> GAEPYGQKKFIEIAGKRMAYIDEGEGDPIVFQHGNPTSSYLWRNIMPHLEGLGRLIACDLIGMGDSDKLSPSGPDRYSYAEHRDYLFALWEALDLGDNVVLVIHDWGSALGFDWANQHRDRVQGIAYMEAIVTPLEWADWPEEVRDIFQGFRSPAGEEMVLENNIFVERVLPGAILRQLSDEEMAEYRRPFLNAGEDRRPTLSWPRQIPIDGEPADVVAIVSDYASWLAESDIPKLFINAEPGAIVTGRMRDFCRSWPNQTEITVKGAHFIQEDSPDEIGAAIAEFVRRLRVAAGV

Haloalkane dehalogenases (HLDs) (EC 3.8.1.5) are hydrolytic enzymes that cleave carbon-halogen bonds in a broad range of halogenated aliphatic compounds, resulting in a corresponding alcohol, a halide ion, and a proton. The tertiary structure of HLDs is comprised of two domains: an α/β-hydrolase core domain and a helical cap domain. HLDs are divided into three subfamilies, HLD-I, HLD-II, and HLD-III, according to the composition of their catalytic residues and the anatomy of the cap domain. Based on the sequences of modern haloalkane dehalogenases from the subfamily II, the most common ancestor of thoroughly characterized enzymes LinB from Sphingobium japonicum UT26 and DmbA from Mycobacterium bovis 5033/66 was in silico predicted, recombinantly produced and structurally characterized.

The ancestral enzyme AncLinB-DmbA was crystallized using the sitting-drop vapor-diffusion method, yielding rod-like crystals that diffracted X-rays to 1.5 Å resolution. The structural organization of AncLinB-DmbA is similar to other HLDs-II subfamily members; it is composed of two compact domains, a cap domain and a main domain. The catalytic triad contains nucleophile D109, catalytic acid E133, and catalytic base H273. W110 and N39 act as halide-stabilizing residues in AncLinB-DmbA. The chloride anion is coordinated by two halide stabilizing residues with distances between the Nε1 atom in W110 and the Nδ1 atom in N39 of 3.29 and 3.37 Å, respectively. The 3D structure of AncLinB-DmbA was superposed with its closely related structures of descendant enzymes LinB and DmbA. As it is shown in Figure 2a the enzyme structure is highly conserved (RMSD of Cα atoms of AncLinB-DmbA and LinB is 0.778 Å and AncLinB-DmbA and DmbA is 0.895 Å), however, some small differences between the structure of ancestral and descendant enzymes were identified. Furthermore, some differences are presented in several loops: the loop near the N-terminus of AncLinB-DmbA forms an additional small helix and another additional helix is formed in AncLinB-DmbA between α3 and β6, which is not presented in DmbA and LinB structures. The AncLinB-DmbA and LinB contain one main tunnel p1 (highlighted in blue) and one slot tunnel p2a, while DmbA has one main tunnel p1 and two slot tunnels p2a and p2b. The radius of the entrance in AncLinB-DmbA is the largest among the descendants: it is ∼2.5 Å, compared to DmbA ∼2.2 Å and LinB ∼1.4 Å. The volume of the active site cavity of AncLinB-DmbA is 460 Å3, which is larger compared to both LinB (406 Å3) and DmbA (375 Å3).> SGNNFEYTLEASKSLRQKPGDSTMTYLNKGQFYPITLKEVSSSEGIHHPISKVRSVIMVVFAEDKSREDQLRHWKYWHSRQHTAKQRCIDIADYKESFNTISNVEEIAYNAISFTWDINDEAKVFISVNCLSTDFSSQKGVKGLPLNIQIDTYSYNNRSNKPVHRAYCQIKVFCDKGAERKIRDEERKQSKRKVSDVKVP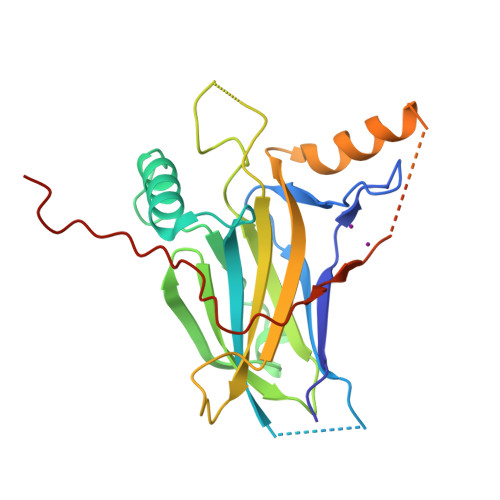LLPSHKRMDITVFKPFIDLDTQPVLFIPDVHFANLQRG>GGTTGGTGTGGTTGG[2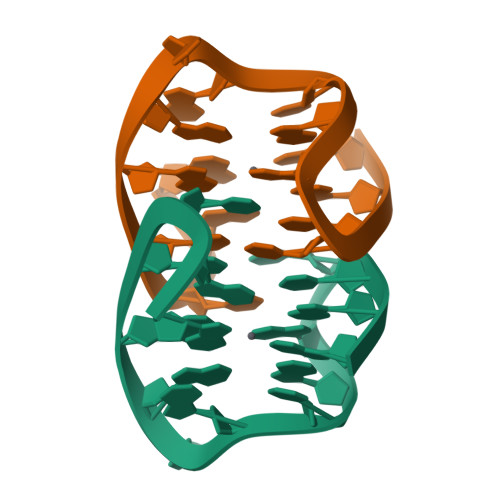x]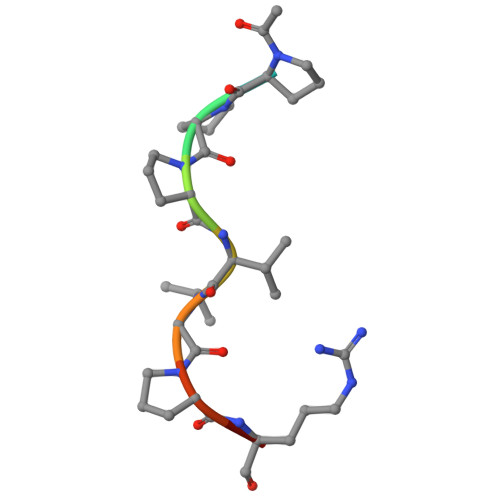> XPPPVGPRR> KGNNCLDAAKACNLDDTCKKYRSAYITPCTTSMSNEVCNRRKCHKALRQFFDKVPAKHSYGMLFCSCRDIACTERRRQTIVPVCSYEERERPNCLSLQDSCKTNYICRSRLADFFTNCQPESRSVSNCLKENYADCLLAYSGLIGTVMTPNYV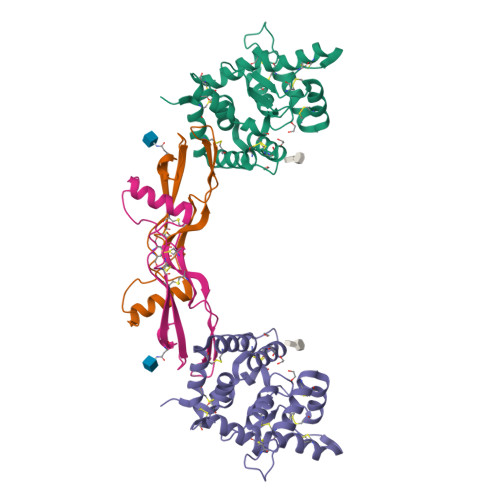DSSSLSVAPWCDCSNSGNDLEDCLKFLNFFKDNTCLKNAIQAFGNGS;> QRGKNRGCVLTAIHLNVTDLGLGYETKEELIFRYCSGSCDAAETTYDKILKNLSRNRRLVSDKVGQACCRPIAFDDDLSFLDDNLVYHILRKHSAKRCGCI>[4x]MFDVIVKNCRLVSSDGITEADILVKDGKVAAISADTSDVEASRTIDAGGKFVMPGVVDEHVHIIDMDLKNRYGRFELDSESAAVGGITTIIEMPITFPPTTTLDAFLEKKKQ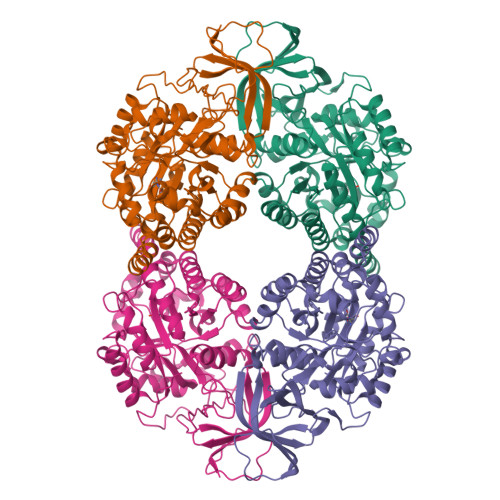AGQRLKVDFALYGGGVPGNLPEIRKMHDAGAVGFKSMMAASVPGMFDAVSDGELFEIFQEIAACGSVIVVHAENETIIQALQKQIKAAGGKDMAAYEASQPVFQENEAIQRALLLQKEAGCRLIVLHVSNPDGVELIHQAQSEGQDVHCESGPQYLNITTDDAERIGPYMKVAPPVRSAEMNIRLWEQLENGLIDTLGSDHGGHPVEDKEPGWKDVWKAGNGALGLETSLPMMLTNGVNKGRLSLERLVEVMCEKPAKLFGIYPQKGTLQVGSDADLLILDLDIDTKVDASQFRSLHKYSPFDGMPVTGAPVLTMVRGTVVAEKGEVLVEQGFGQFVTRRNYEASK>MEAEQRPAAGASEGATPGLEAVPPVAPPPATAASGPIPKSGPEPKRRHLGTLLQPTVNKFSLRVFGSHKAVEIEQERVKSAGAWIIHPYSDFRFYWDLIMLLLMVGNLIVLPVGITFFKEENSPPWIVFNVLSDTFFLLDLVLNFRTGIVVEEGAEILLAPRAIRTRYLRTWFLVDLISSIPVDYIFLVVELEPRLDAEVYKTARALRIVRFTKILSLLRLLRLSRLIRYIHQWEEIFHMTYDLASAVVRIFNLIGMMLLLCHWDGCLQFLVPMLQDFPPDCWVSINHMVNHSWGRQYSHALFKAMSHMLCIGYGQQAPVGMPDVWLTMLSMIVGATCYAMFIGHATALIQSLDSSRRQYQEKYKQVEQYMSFHKLPADTRQRIHEYYEHRYQGKMFDEESILGELSEPLREEIINFTCRGLVAHMPLFAHADPSFVTAVLTKLRFEVFQPGDLVVREGSVGRKMYFIQHGLLSVLARGARDTRLTDGSYFGEICLLTRGRRTASVRADTYCRLYSLSVDHFNAVLEEFPMMRRAFETVAMDRLLRIGKKNSILQRKRSEPSPGSSGGIMEQHLVQHDRDMARGVRGRAPSTGAQLSGKPVLWEPLVHAPLQAAAVTSNVAIALTHQRGPLPLSPDSPATLLARSAWRSAGSPASPLVPVRAGPWASTSRLPAPPARTLHASLSRAGRSQVSLLGPPPGGGGRRLGPRGRPLSASQPSLPQRATGDGSPGRKGSGSERLPPSGLLAKPPRTAQPPRPPVPEPATPRGLQLSANM[4x]

pmcHyperpolarization-Activated Cyclic Nucleotide-gated (HCN) channels represent a class of unique voltage-gated cation channel that are activated by membrane hyperpolarization and modulated by cyclic nucleotide and membrane lipids. HCN channels play a major role in neuronal excitability and cardiac pacemaker activity and have emerged as attractive targets for the treatment of various heart and central nervous system disorders, including heart failure, depression, neuropathic pain, and epilepsy. The recent cryo-EM structures of HCN1 (31) and HCN4 (32) unveiled a tetrameric topology, with an intracellular N-terminal domain, including the HCN domain, six transmembrane domains (TMDs), and C-terminal domain, including C-linkers and cyclic nucleotide-binding domain (CNBD), which contains the binding site of cAMP. To understand the mechanism of ligand and lipid sensing by HCN channels, we determined two cryo-EM structures of HCN3:ligand-free and cAMP-bound structures.

To investigate the conformational changes that HCN modulators induce, we performed cryo-EM analyses of full-length human HCN3 in physiological conditions which bind with cAMP. The overall structure of cAMP-HCN3 showed high similarity to the apo-HCN3 structure (RMSD = 0.529). The TMDs of cAMP-bound HCN3 closely resemble those of apo-HCN3 conformation, and the structure of TMD of HCN3 in the presence of cAMP was similar to that in its absence, indicating that addition of cAMP alone is insufficient to open the channel. The superimposition of a single subunit from the apo- and cAMP-bound structures shows that cAMP-binding causes rigid body movements of CNBD domains, resulting in a 10 Å closure of the cleft between C helix and β strand 4. Secondly, the density of CHS was not observed in cAMP-bound structures, which is consistent with the idea that CHS represents an inactivating lipid. In the cAMP-HCN3 structure, we observe a strong density that bridges the C helix and β strand 4 at the site where cAMP is expected to bind. The cAMP-binding pocket is located at a cleft between the C helix, P helix, and β strand 4, which together form the CNBD of HCN3. The cAMP-HCN3 structure reveals that the residue R543 on the C helix forms hydrogen bonds and cation–π interactions with the AMP of cAMP, primarily stabilizing the CNBD domain. The phosphate group of cAMP is pointed inward within the cAMP-binding cleft and is accommodated by residues R463, C495, and T503. Specifically, the C helix in the CNBD shifts 30 degrees.> VADSASTVTNEFSADHPFIYVIRHVDGKIL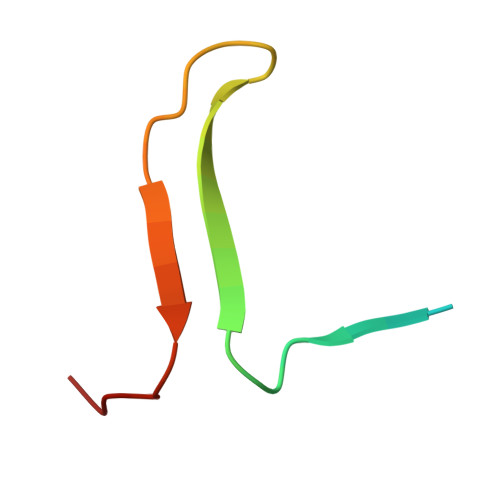FVGRYSSPTTN Here we present the structural and functional studies of SCARB2, a functional receptor of the important human enterovirus 71 (EV71). SCARB2 is responsible for attachment as well as uncoating of EV71. SCARB2 is ubiquitously expressed and serves as a common receptor for all clinically isolated EV71 strains, CVA16, CVA7 and CVA14. SCARB2 (residues 37–430) consists of three domains arranged in a “Kidney” shape.

To gain an understanding of the molecular basis of SCARB2-mediated uncoating of EV71 under acidic conditions, we solved the crystal structures of the ectodomain of SCARB2 under both neutral (pH 7.5) (hereafter denoted as nSCARB2) and acidic conditions (pH 4.8) (hereafter denoted as aSCARB2). In contrast the elucidation of the structure of nSCARB2 (pH 7.5) at higher resolution (3.0 Å) and its comparison with aSCARB2 enabled us to visualize a pivotal conformational change in SCARB2 induced by pH that has implications for the function of the receptor. In contrast, at pH 7.5, the re-positioning of α5 in vicinity of α4 and α7 blocks the membrane-distal end of the tunnel, decreasing its void volume from 4,867 Å3 to 4,554 Å3 [calculated by program HOLLOW]. Thus in nSCARB2, α5 (residues 157–164) adopts a short helical conformation. Helices α4, α5 and α7 are held together in a compact cluster by hydrophobic interactions involving residues W146, L152, I156, Y163 of α4–α5 and I184, L187, I188, F191, I195 from α7. Under neutral conditions, a cap closes the entrance of the lipid-transfer tunnel of SCARB2. Amongst these multiple sites, based on the contour of the electron density and prior knowledge that lysosomal enzymes are often modified with Man9GlcNA2-P, the glycan at N325 of nSCARB2 was modeled as Man8GlcNA2. N325 is located at the bottom of a cleft formed between helices α11 and α12. Man8GlcNA2 protrudes to the surface out of this chasm and stations itself in vicinity of the cap. Notably, the sugar moieties adjacent to α4 and α5 are stabilized by P314, E145 and H150.

>IEKKIVLRNGTEAFDSWEKPPLPVYTQFYFFNVTNPEEILRGETPRVEEVGPYTYRELRNKANIQFGDNGTTISAVSNKAYVFERDQSVGDPKIDLIRTLNIPVLTVIEWSQVHFLREIIEAMLKAYQQKLFVTHTVDELLWGYKDEILSLIHVFRPDISPYFGLFYEKNGTNDGDYVFLTGEDSYLNFTKIVEWNGKTSLDWWITDKCNMINGTDGDSFHPLITKDEVLYVFPSDFCRSVYITFSDYESVQGLPAFRYKVPAEILANTSDNAGFCIPEGNCLGSGVLNVSICKNGAPIIMSFPHFYQADERFVSAIEGMHPNQEDHETFVDINPLTGIILKAAKRFQINIYVKKLDDFVETGDIRTMVFPVMYLNESVHIDKETASRLKSMIN[2x]>MGHHHHHHENLYFQGHMASGSDAVSPELRSRALTIVVLGASGDLAKKKTFPALFQLYCNGMLPRDVNILGYARSTMEDVEKWKKDTLAGFFTRLDERGCHVGNFLRRISYMTGSYDRDEDFARLNERILRMEEAFQGPEKGGNRLFYLALPPSVFVGVCRGLSKGAMQKPELGWVRLIVEKPFGRDTETSEQLSNQLKPLFNERQVFRIDHYLGKEMVQNIIVTRFANRVFSALWNSNSIACVQITFKEKIGTAGRGGYFDSIGIIRDVIQNHLTQILSLLTMEKPR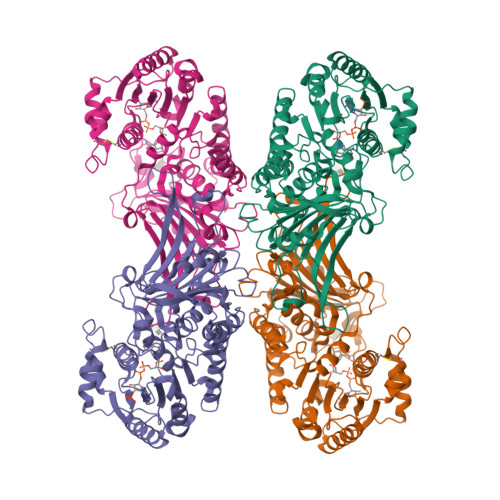SLSAEDIRDEKVQVLRQVVPANPAECVLGQYTASADGSTPGYLDDPSVPKGSHCPTFAVLRLHVNNDRWHGVPFIIRAGKALEERLLDIRIQFKDEIRPFGESTQRNELVIRAQPSEAMYLKLTAKTPGLLNDTHQTELDLTYERRYDVTLPDAYESLIHEALLGNSTNFVRVDELDAAWRIYTPLLHAIDRGEVKVLPYAAGSCGPEEAQEFIRISGYKTT[3x]>ASLAADTPTACCFSYTSRQIPQNFIADYF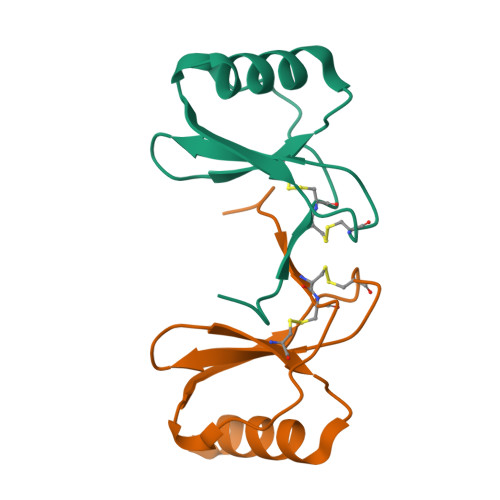ETSSQCSKPGVIFLTKRSRQVCADPSEEWVQKYVSDLELSA[5x]>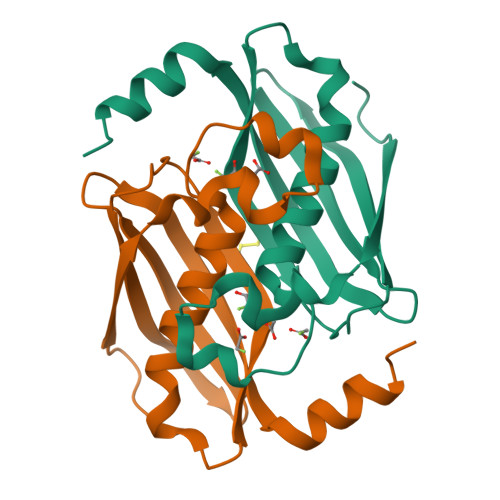[2x]GTGAMKDGMRVGERFTHDFVVPPHKTVRHLYPESPEFAEFPEVFATGFMVGLMEWACVRAMAPYLEPGEGSLGTAICVTHTAATPPGLTVTVTAELRSVEGRRLSWRVSAHDGVDEIGSGTHERAVIHLEKFNAKVRQKTPAG>MGHHHHHHSIETDRVSKEFIEFLKTFHKTGQEIYKQTKLFLEGMHYKRDLSIEEQSECAQDFYHNVAERMQTRGKVPPERVEKIMDQIEKYIMTRLYKYVFCPETTDDEKKDLAIQKRIRALRWVTPQMLCVPVNEDIPEVSDMVVKAITDIIEMDSKRVPRDKLACITKCSKHIFNAIKITKNEPASADDFLPTLIYIVLKGNPPRLQSNIQYITRFCNPSRLMTGEDGYYFTNLCCAVAFIEKLDAQSLNLSQEDFDRYMSGQTSPRKQMYKNLDLLSQLNERQERIMNEAKKLEKDLIDWTDGI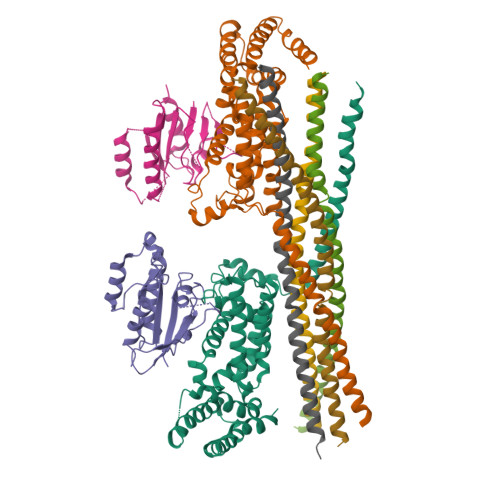AREVQDIVEK[2x];>[2x]SGNKICQFKLVLLGESAVGKSSLVLRFVKGQFHEFQESTIGAAFLTQTVCLDDTTVKFEIWDTAGQERYHSLAPMYYRGAQAAIVVYDITNEESFARAKNWVKELQRQASPNIVIALSGNKADLANKRAVDFQEAQSYADDNSLLFMETSAKTSMNVNEIFMAIAKKLPKN;>METRDQVKKLQLMLRQANDQLEKTMKDKQELEDFIKQSSEDSSHQISALVLRAQASEILLEELQQGLSQAKRDVQEQMAVLMQSREQVSEEL[4x]>[6x]MEKKFMRESKAIKTTRVFPNDLNNHQTLFGGKLLAEIDSIASIAAARHSRKHCVTASIDSVDFLTPIHQADSVCYEAFVCY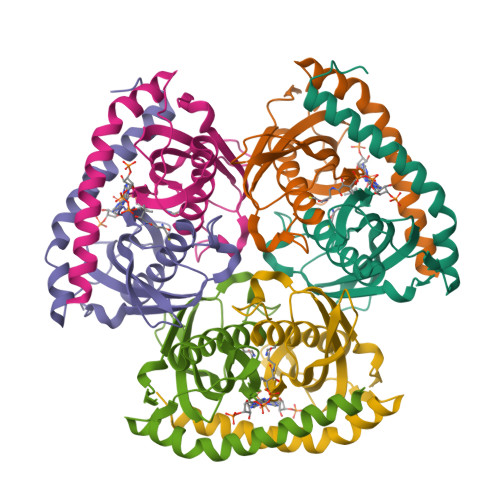TGKSSMEVFVKVIAENLLAGERRIAATCFITFVAIKDGKPSSVPQVLPETQEEHWLHKTGLERAENRKKGRLKSKEMAEVLTLSKPWNILEHHHHHH> HHHHHHMRVLGLNGWPRDFNDASAALLVDGRIAAFAEEERFTRKKHGYNTAPVQAAAFCLAQAGLTVDDLDAVAFGWDLPAMYRERLGGWPHSDSEALDILLPRDVFPRRTDPPLHFVQHHLAHAASAYYFSGEDRGAVLIVDGQGEEECVTLAHAEGGKITVLDTVPGAWSLGFFYEHVSEYTGLGGDNPGKLMGLAAHGTTVDETLSAFAFDSDGYRLNLIDPQARDPEDWDEYSVTERAWFAHLER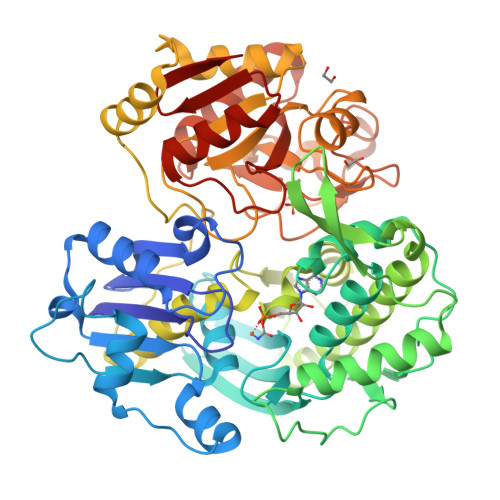IYRLPPNEFVRRYDPAKGRVVRDTRRDPYEYRDLAATAQAALERAVFGLADSVLARTGERTLFVAGGVGLNATMNGKLLTRSTVDKMFVPPVASDIGVSLGAAAAVAVELGDRIAPMGDTAAWGPEFSPDQVRAALDRTGLAYREPANLEREVAALIASGKVVGWAQGRGEVGPRALGQRSLLGSAHSPTMRDHINLRVKDREWWRPFAPSMLRSVSDQVLEVDADFPYMIMTTKVRAAYAERLPSVVHEDWSTRPQTVTEASNPRYHRMLTELGDLVGDPVCLNTSFNDRGEPIVSSPADALLTFSRLPIDALAVGPYLVTKDLRH>GSHMALSPGAGKITDKIAMLGEGGVGKTSLTVNLTKHVFSETYDPTLEDSYRRQCVIDGIPSHLEILDTAGQEEYGALREQWIRQNELFVIVFDVTRRSSFEAAERLFEEVIQTKRKLDETRRHPGDRHPDDLPFAPSLVVLVGNKCDLDTRREVGTLEG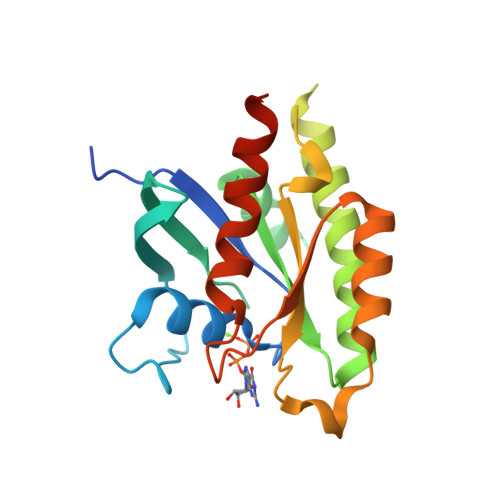SSLAKKLGCGFVETSAKLGTNVEEAFFSVVRADRRRKREVTDEEQR[2x]>UAUGGAAGAGGCGGUUGGUAU[2x]

G-quadruplexes form in G-rich DNA or RNA when four guanines form hydrogen bonds to create Hoogsteen geometry and form a tetrad. These tetrad structures are further stabilized by a monovalent cation, usually potassium, and π-stacks forming a stable quadruplex. In this work, we report the crystal structure of a viral genomic RNA G-quadruplex, which was derived from the sequence in the NS5 gene of WNV. The NS5-B quadruplex sequence remains highly conserved with minor changes in loop residues across a diverse set of both mosquito-borne and tick-borne Orthoflavivirus members.

To improve NMR peak resolution further, we designed a modified RNA sequence, NS5-B M1 with G→A substitutions near the 5ʹ and 3ʹ termini. The x-ray crystal structure of NS5-B M1 was resolved to 1.97 Å and contains two non-equivalent quadruplex copies per asymmetric unit, Chains A and B, packed head-to-head. Each monomer contains two G tetrads arranged in a right-handed parallel strand configuration. In both structures, the first tetrad (α) is composed of nucleotides G4-G10-G13-G17, and the second tetrad (β) is formed by G5-G11-G14-G18. A third set of stacked bases forms a triad (γ) composed of G8-U15-U19 and is further capped by the A6 ∙ A20 dyad. The G tetrads have both north and south sugar pucker conformations, and the bases adopt an anti-conformation. A K+ ion is coordinated between the α- and β-tetrads in both chains, and NH4+ ions are present between the β-tetrad and γ-triad in both Chain A & Chain B as well as at the interface between the copies. Another surprising structural observation is that two of the loop residues, A9 and C12, interact directly with the α-tetrad. Two distinct C12 conformations were observed in Chains A and B of the structure. In the “flipped in” position (Chain A), C12 forms two nonconical C12 ∙ G10, N3-amino, amino-N3 hydrogen bonds.> MKQDSASNATYTVDCEDYVHVVEFNPFDSGEAGSLLAYGGISYVVIASCRFQEEDSTVEGIEFKTLKTFHHGERVVAIAWSPETRCDALLPLLRFATAAGDKKIRIFTSDFQDKNEYKVIEGHSGYINDLVFCSPEGTDIASVGDDHTCRIWDLDGKQIAMFILRSPGMSVAWHPE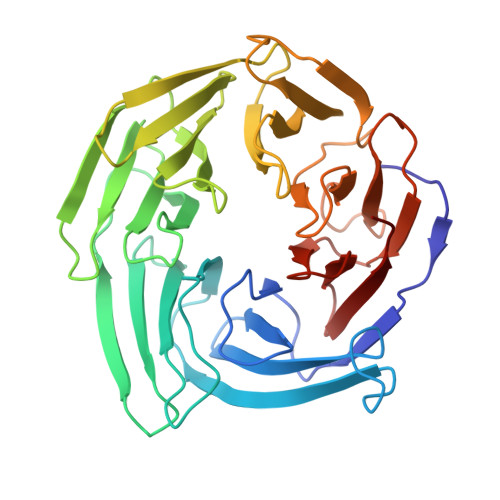GAFKLMVAEKTGTIRFYDLTTHQAILSLESVQVPLMSADWCVRNTLRIGAVAGNDWIIWEMPRSSYPQDNKPAHADRARMFRWSKCNENVFATTGYPGKMKSQIAIHHLAHPQPILIGTAPVGSGLSWHRRLPLCVVGGYRKLFFWLTEM> MAHHHHHHMSFNIFIASDHTGLTLKKIISEHLKTKQFNVVDLGPNYFDANDDYPDFAFLVADKVKKNSDKDLGILICGTGVGVCMAANKVKGVLAALVVSEK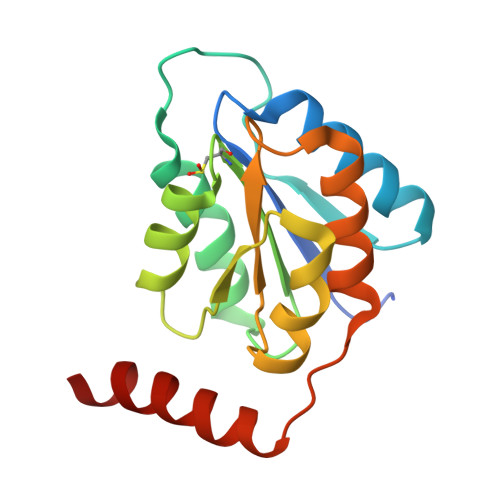TAALARQHDNANVLCLSSRFVTDSENIKIVDDFLKANFEGGRHQRRIDKIIRYEKETE5-methoxy-1,3-benzothiazol-2-amine | C8 H8 N2 O S | 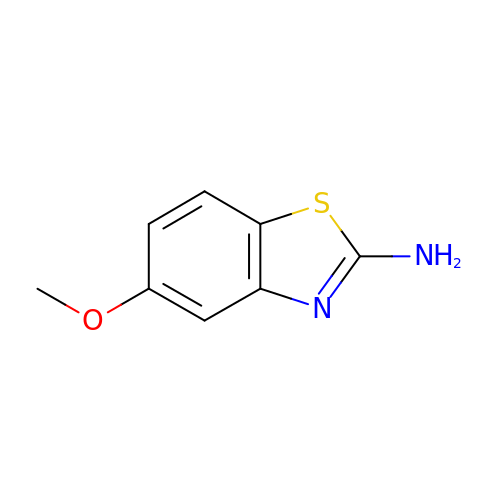OMIHQJBWAPWLBO-UHFFFAOYSA-N> MPLDETNNESYRYLRSVGNTWKFNVEDVHPKMLERLYKRFDTFDLDTDGKMTMDEIMYWPDRMRQLVNATDEQVEKMRAAVHTFFFHKGVDPVNGLKREDWVEANRVFAEAERERERRGEPSLIALLSNAYYDVLDDDGDGTVDVEELKTMMK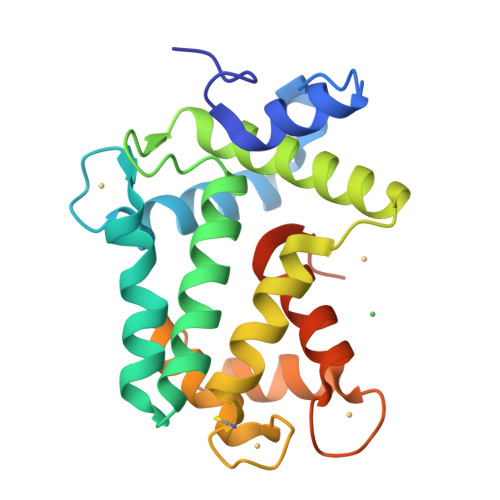AFDVPQEAAYTFFQKADTDKTGKLERPELVHLFRKFWMEPYDPQWDGVYAYKY>MSSRLLPPNRSSLERSLGDVLPAELPVPLRELHDPARCEAALLPYLAWTRSVDRWDPDWSDEAKRNAVATSFVLHQRKGTLTALRQVVEPIGALSEVTEWWQRSPTGVPGTFEITVDVSDRGIDEGTVLELERLLDDVRPVSRHLTRLDLRITPVIRSRHGLAVTDGDTLEIFPWKQ[6x];>MIGMDRRSGLPLSGLAHLKQSVEDILTTPLGSRRMRPEYGSKLRRMVDMPVSEGWKSAVQAEVARSLGRWEPRIGLSAVRVVAVVDGRVDLLLSGVFEGENINMEVSA[6x];>[6x]MATTCRTADGDMLDSLCYHVYGHLLGCVEATLDANPGLADEQQPFRAGLLISFPDMPVVNVEQVRLWD;>MIIDL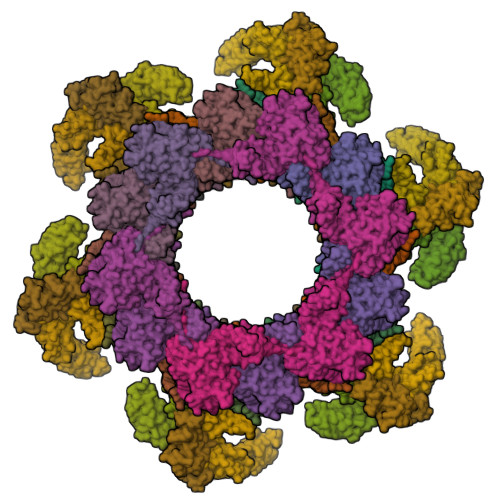SQLPEPEVIENLDFETIYQELLGDFREAMAGEWTAEVESDPVLKLLQLAAYRELLLRARINDAARAVMLAYASGADLDQIGAGFNVQRLLIRPAQPEAVPPVEAQYESDKSLRNRIQLAFEQLSVAGPRNAYIAHALGADGRVADASATSPAPCEVLISVLGVEGNGQAPEAVLQAVRLALNAEDVRPVADRVTVRSAGIVPYQVKAQLYLFPGPEAELIRAAAEASLRDYISAQRRLGRDIRRSALFATLHVEGVQRVELQEPAADVVLDETQAAYCTGYAITLGGVDE[12x];>MSFFHGVTVTNVDIGARTIALPASSVIGLCDVFTPGAQASAKPNVPVLLTSKKDAAAAFGIGSSIYLACEAIYNRAQAVIVAVGVETAETPEAQASAVIGGISAAGERTGLQALLDGKSRFNAQPRLLVAPGHSAQQAVATAMDGLAEKLRAIAILDGPNSTDEAAVAYAKNFGSKRLFMVDPGVQVWDSATNAARNAPASAYAAGLFAWTDAEYGFWSSPSNKEIKGVTGTSRPVEFLDGDETCRANLLNNANIATIIRDDGYRLWGNRTLSSDSKWAFVTRVRTMDLVMDAILAGHKWAVDRGITKTYVKDVTEGLRAFMRDLKNQGAVINFEVYADPDLNSASQLAQGKVYWNIRFTDVPPAENPNFRVEVTDQWLTEVLDVA[24x]>[3x]MPFITVGQENSTSIDLYYEDHGTGTPVVLIHGFPLSGHSWERQSAALLDAGARVITYDRRGFGQSSQPTTGYDYDTFAADLNTVLETLDLQDAVLVGFSMGTGEVARYVSSYGTARIAAVAFLASLEPFLLKTDDNPDGAAPQEFFDGIVAAVKADRYAFYTGFFNDFYNLDENLGTRISEEAVRNSWNTAASGGFFAAAAAPTTWYTDFRADIPRIDVPALILHGTG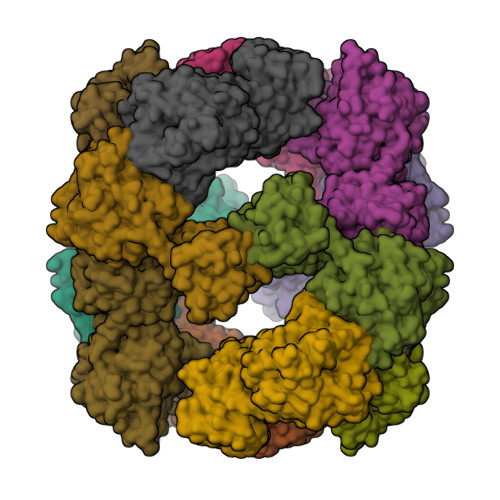DRTLPIENTARVFHKALPSAEYVEVEGAPHGLLWTHAEEVNTALLAFLAKAQEAQKQKLLTEVETYVLSIIPSGPLKAEIAQRLEDVFAGKNTDLEVLMEWLKTRPILSPLTKGILGFVFTLTVPSERGLQRRRFVQNALNGNGDPNNMDKAVKLYRKLKREITFHGAKEISLSYSAGALASCMGLIYNRMGAVTTEVAFGLVCATCEQIADSQHRSHRQLEHHHHHH> MSKRIALFPALLLALLVIVATALTWMNFSQALPRSQWAQAAWSPNINVIEQMIFHYSLLPRLAISLLVGAGLGLVGVLFQQVLRNPLAEPTTLGVATGAQLGITVTTLWAIPGAMASQFAALAGACVVGLIVFGVAWGKRLSPVTLILAGLVVSLYCGAINQLLVIFHHDQLQSMFLWSTGTLTQTDWGGVERLWPQLLGGVMLTLLLLRPLTLMGLDDGVARNLGLALSLARLAALSLAIVISALLVNAVGIIGFIGLFAPLLAKMLGARRLLPRLMLASLIGALILWLSDQIILWLTRVWMEVSTGSVTALIGAPLLLWLLPRLRSISAPDMKVNDRVATERQHVLAFALAGGVLLLMAVVVALSFGRDAHGWTWASGALLDDLMPWRWPRIMAALFAGVMLAVAGCIIQRLTGNPMASPEVLGISSGAAFGVVLMLFLVPGNAFGWLLPAGSLGAAVTLL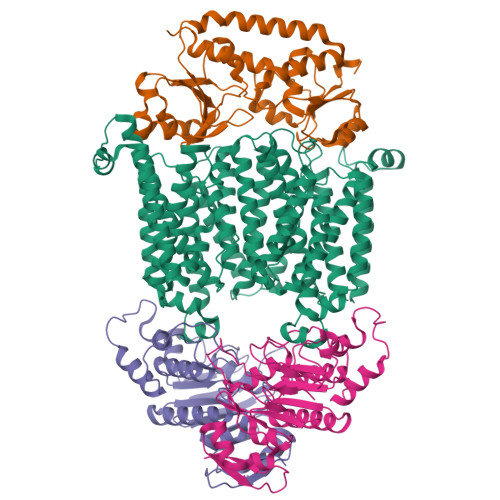IIMIAAGRGGFSPHRMLLAGMALSTAFTMLLMMLQASGDPRMAQVLTWISGSTYNATDAQVWRTGIVMVILLAITPLCRRWLTILPLGGDTARAVGMALTPTRIALLLLAACLTATATMTIGPLSFVGLMAPHIARMMGFRRTMPHIVISALVGGLLLVFADWCGRMVLFPFQIPAGLLSTFIGAPYFIYLLRKQSRHHHHHHHH;>[2x]MQEYTNHSDTTFALRNISFRVPGRTLLHPLSLTFPAGKVTGLIGHNGSGKSTLLKMLGRHQPPSEGEILLDAQPLESWSSKAFARKVAYLPQQLPPAEGMTVRELVAIGRYPWHGALGRFGAADREKVEEAISLVGLKPLAHRLVDSLSGGERQRAWIAMLVAQDSRCLLLDEPTSALDIAHQVDVLSLVHRLSQERGLTVIAVLHDINMAARYCDYLVALRGGEMIAQGTPAEIMRGETLEMIYGIPMGILPHPAGAAPVSFVY;> MSGLPLISRRRLLTAMALSPLLWQMNTAHAAAIDPNRIVALEWLPVELLLALGIVPYGVADTINYRLWVSEPPLPDSVIDVGLRTEPNLELLTTMRPSFMVWSAGYGPSPEMLARIAPGRGFNFSDGKQPLAMARKSLTEMADLLNLQSAAETHLAQYEDFIRSMKPRFVKRGARPLLLTTLIDPRHMLVFGPNSLFQEILDEYGIPNAWQGETNFWGSTAVSIDRLAAYKDVDVLCFDHDNSKDMDALMATPLWQAMPFVRAGRFQRVPAVWFYGATLSAMHFVRVLDNAIGGKA>PPYTVVYFPVRGRCAALRMLLADQGQSWKEEVVTVETWQEGSLKASCLYGQLPKFQDGDLTLYQSNTILRHLGRTLGLYGKDQQEAALVDMVNDGVEDLRCKYISLIYTNYEAGKDDYVKALPGQLKPFETLLSQNQGGKTFIVVDQISFADYNLLDLLLIHEVLAPGCLDAFPLLSAYVGRLSARPKLKAFLASPEYVN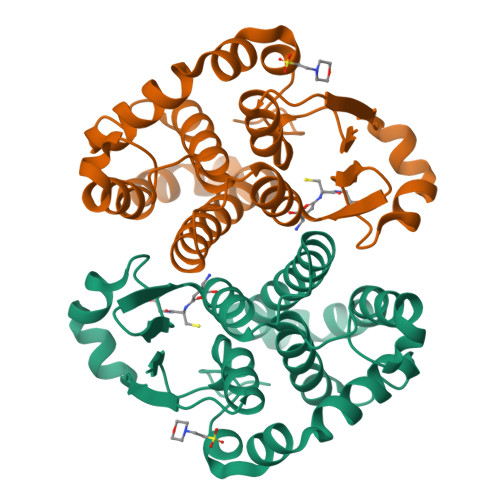LPINGNGKQ[2x]> ESGALPKEAVVQIRLTKKGMIEEKKVTVQELRELYLSGEYTIEIDTPDGYQTIGKWFDKGVL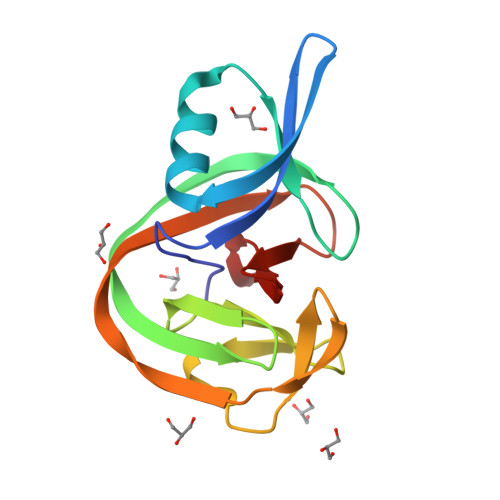SMVRVATATYETVCAFNHMIQLADNTWVQACELDVGVDIQTAAGIQPVMLVEDTSDAECYDFEVMHPNHRYYGDGIVSHASGK>MQGKVALEEHFAIPETLQDSAGFVPGDYWKELQHRLLDIQDTRLKLMDAHGIETMILSLNAPAVQAIPDRRKAIEIARRANDVLAEECAKRPDRFLAFAALPLQDPDAATEELQRCVNDLGFVGALVNGFSQEGDGQTPLYYDLPQYRPFWGEVEKLDVPFYLHPRNPLPQDSRIYDGHPWLLGPTWAFAQETAVHALRLMASGLFDEHPRLNIILGHMGEGLPYMMWRIDHRNAWVKLPPRYPAKRRFMDYFNENFHITTSGNFRTQTLIDAIL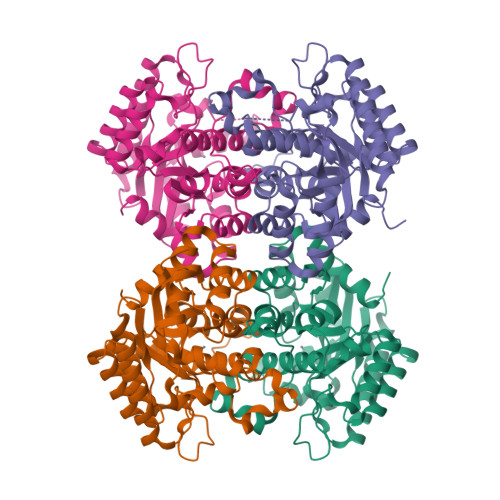EIGADRILFSTDWPFENIDHASDWFNATSIAEADRVKIGRTNARRLFKLDGA[4x]>ARTVVLITGCSSGIGLHLAVRLASDPSQSFKVYATLRDLKTQGRLWEAARALACPPGSLETLQLDVRDSKSVAAARERVTEGRVDVLVCNAGLGLLGPLEALGEDAVASVLDVNVVGTVRMLQAFLPDMKRRGS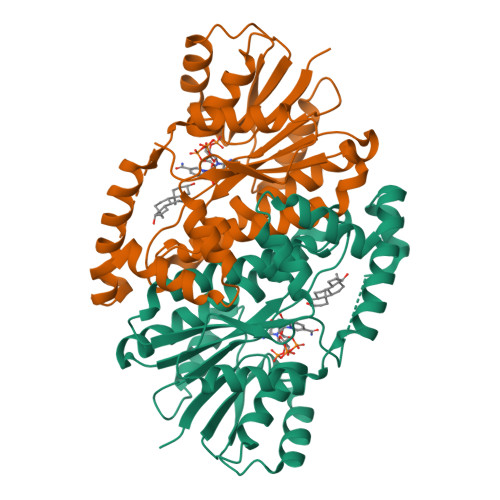GRVLVTGSVGGLMGLPFNDVYCASKFALEGLCESLAVLLLPFGVHLSLIECGPVHTAFMEKVLGSPEEVLDRTDIHTFHRFYQYLAHSKQVFREAAQNPEEVAEVFLTALRAPKPTLRYFTTERFLPLLRMRLDDPSGSNYVTAMHREVFGDVPAKAEAGAEAGGGAGPGAEDEAGRSAVGDPELGDPPAAPQ[2x]2,3,4-TRIMETHYL-1,3-THIAZOLE | C6 H10 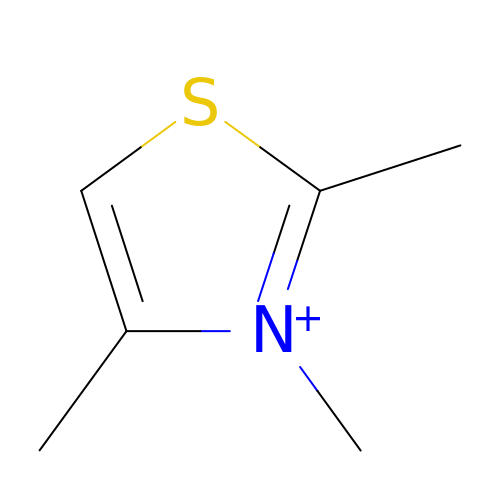N S | UHOYCVRPRYFLFR-UHFFFAOYSA-N>MRGSHHHHHHENLYFQGSPRWILGDKFDTVFPHKGSLKVLWESRWKFACSKSVYPFHDGSIEDFEPIFNHLISKNINDAASDEYTQAFLPTASALEEKAAQALQAGKHEEASNLLCRAAVVYRISRFPYVDITKPNSIKRVAFERQKQAYLKATSLWTQPIREVTVPHTYRTGNDGAHIPIYIRTPAGADQSNPVPIVLIMTGLDGYRPDNSQRTHEILARGWAAVVAEIPGTADCPADPADPASPDRLWDSVLSYLDQRPELNTAKMVVWGLSAGGYYAIRAAHTHRDRLLGAIAHGPGCHYYLDPEWLAKVNDHEYPFEITAAWATKHGYKTVEEFVAGAQKKFSLVETGIVDQPSCRLL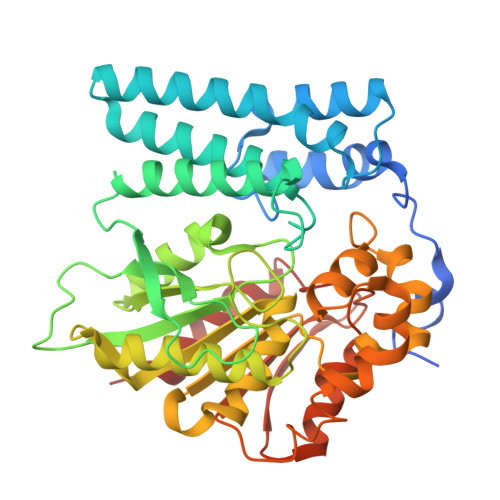LLNGVDDGVVPIEDCLVLFEHGSPKEGRFYKGLPHMGYPNSLPVSYEWLEQVLASPSKTKN[4x]> GSPPNWQQLVSREVLLGLKPCEIKRQEVINELFYTERAHVRTLKVLDQVFYQRVSREGILSPSELRKIFSNLEDILQLHIGLNEQMKAVRKRNETSVIDQIGEDLLTWFSGPGEEKLKHAAATFCSNQPFALEMIKSRQKKDSRFQTFVQDAESNPLCRRLQL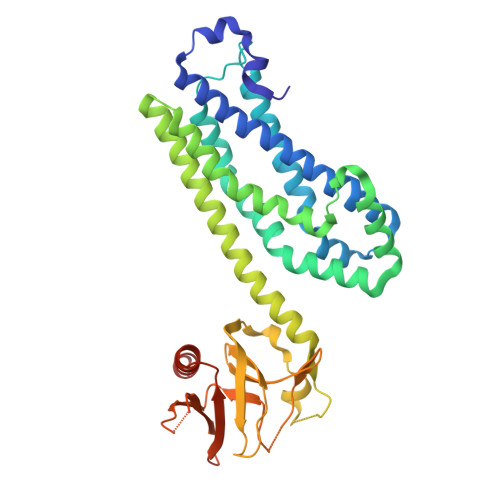KDIIPTQMQRLTKYPLLLDNIAKYTEWPTEREKVKKAADHCRQILNFVNQAVKEAENKQRLEDYQRRLDTSSLKLSEYPNVEELRNLDLTKRKMIHEGPLVWKVNRDKTIDLYTLLLEDILVLLQKQDDRLVLRCHSKILASTADSKHTFSPVIKLSTVLVRQVATDNKALFVISMSDNGAQIYELVAQTVSEKTVWQDLICRMAASVKEQSVDGGHHHHHH methyl 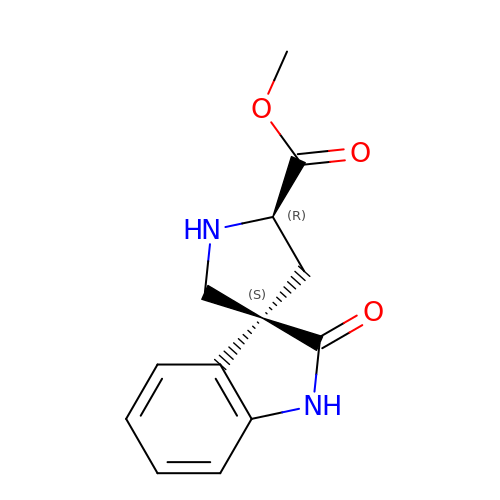(3S,5'R)-2-oxo-1,2-dihydrospiro[indole-3,3'-pyrrolidine]-5'-carboxylate | C13 H14 N2 O3 | WBRZAMFFUKWSQR-ZWNOBZJWSA-N> 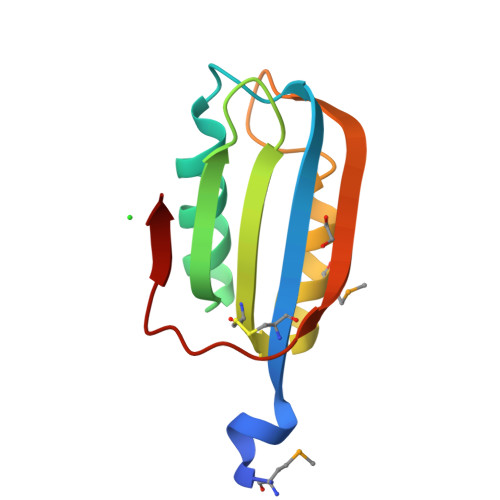SNAMTQKEKNETCIHVTVSGKVQGVFFRESVRKKAEELQLTGWVKNLSHGDVELVACGERDSIMILTEWLWEGPPQAAVSNVNWEEIVVEDYSDFRVR> MKLIAESGSTKTEWSLVEGEHLIQRVFTEGLNPFFQTRREISRSIRLGLPDSFFKRKLEQVFFYGAGCTSAEKKSVVEASLVAQFKTPAYVESDLLAAARGLFQHDSGIACILGTGSNSCFYDGHVIVKNVRAGGYILGDEGSGAALGKQFLSDVLKKLAPQVLIDDFFEKYDLTPHDVMDVVYNRPFPNRFLAEQSCFLADYLRLDYVKGLLLSNLRSFFLRNVMQYDYLNYPIRFVGSVAYNYADLLHQVGKEFGVELSVVEETPMGGLIKYHAFPPDDPES

Unlike other bacteria, the pathogenic Tannerella forsythia, a member of the red complex group of bacteria associated with the late stages of periodontitis, lacks biosynthetic pathways for MurNAc production and therefore obtains MurNAc from the environment. Sugar kinases play a crucial role in the MurNAc recycling process, activating the sugar molecules by phosphorylation. MurK and K1058 are two sugar kinases of the cell wall recycling system of T. forsythia, sharing a sequence identity of 44% and separated by a single PGN-scavenging operon within the genome. Structural and sequence data showed that MurK and K1058 both belong to the group of ribonuclease H-like kinases and are members of the ASKHA (acetate and sugar kinase/hsc70/actin) superfamily.

Based on genomic sequence analysis, a second putative MurNAc kinase, termed K1058, was identified in T. forsythia, sharing a sequence similarity of 44% to MurK. We were able to obtain structures of the apo enzyme (K1058apo) and K1058 in complex with MurNAc (K1058/MurNAc). K1058 crystallized in a tetragonal space group (termed K1058apo) with a single protomer in the ASU. The biological corresponding dimer interface as is observed for MurKapo results from the application of the crystallographic two-fold axis. A superposition showed a close relationship between K1058 and MurK, with an observed Cα-RMSD value of 2.1 Å over the total protein length. Initial attempts of soaking MurNAc into MurKapo or K1058apo crystals with or without an ATP analog failed, probably due to an induced fit accompanying MurNAc binding.>SNAMNFFTSPFSGIPLDQQVTNPNIIVGKHSYYSGYYHGHSFDDCVRYLHPERDDVDKLVIGSFCSIGSGAVFMMAGNQGHRSDWISTFPFFYQDNDNFADARDGFTRSGDTIIGHDVWIGTEAMIMPGVKIGHGAIIASRSVVTKDVAPYEVVGSNPAKHIKFRFSDVEIAMLLEM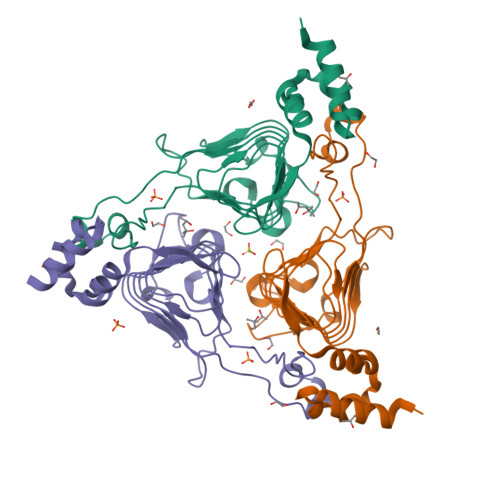AWWNWPESWLKESMQSLCSSDIEGLYLNWQSKART[3x]>MAQLALQMSSLGVEGEGIWLALGTIGMLLGMLYFIADGLDVQDPRQKEFYVITILIPAIAAASYLSMFFGFGLTEVSLANGRVVDVYWARYADWLFTTPLLLLDIGLLAGASQRDIGALVGIDAFMIVTGLVATLTKVVVARYAFWTISTISMVFLLYYLVAVFGEAVSDADEDTRSTFNALRNIILVTWAIYPVAWLVGTEGLALTGLYGETLLFMVLDLVAKVGFGFILLRSRAIMGGGSEPTPSAQETAADHHHH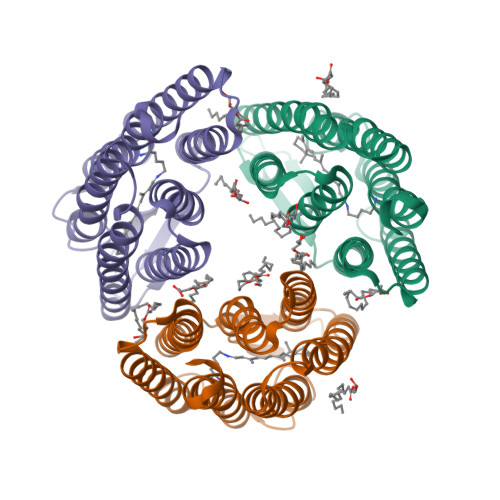HHLEHHHHHH[3x]> MWYKYFSKQSWNLRVWRKANLKYNQDDFGMTQPKYIARFGDFRFRLVRTEGALRGCMFFVGFGCFSIINYLYGRYGYIINESSQKRAAQDLLDNDMAADKILFKNRVGAPTRPLRSLDDMMAFLSGSATY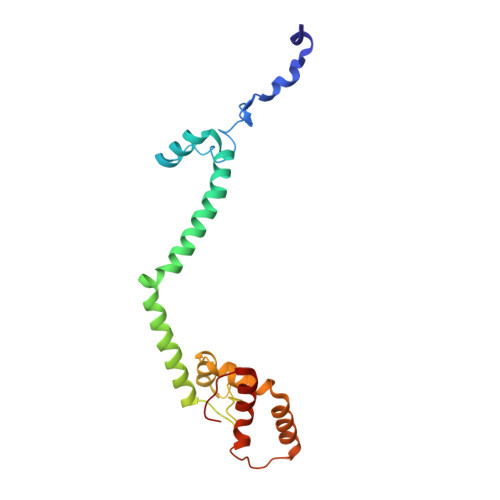DQLADYASYNHAMDVNQDQQAGLDSWMSEKDKNMVKYYQRSLGKKVEGI>MARKYFVAANWKCNGTLESIKSLTNSFNNLDFDPSKLDVVVFPVSVHYDHTRKLLQSKFSTGIQNVSKFGNGAYTGEVSAEIAKDLNIEYVIIGHSERRKYFHETDEDVREKLQASLKNNLKAVVCFGESLEQREQNKTIEVITKQVKAFVDLIDNFDNVILVYEPLWAIGTGKTATPEQAQ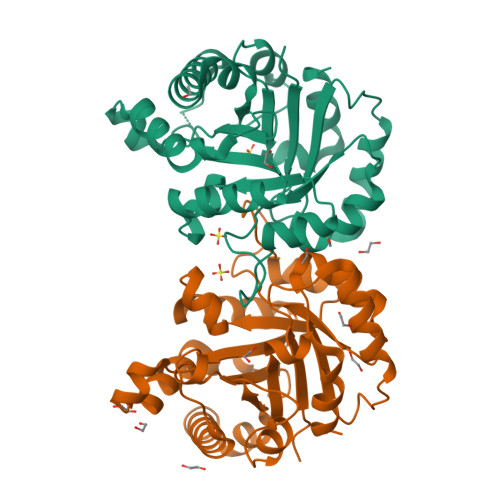LVHKEIRKIVKDTCGEKQANQIRILYGGSVNTENCSSLIQQEDIDGFLVGNASLKESFVDIIKSAM[2x]>PMFIVNTNVPRASVPDGFLSELTQQLAQATGKPPQYIAVHVVPDQLMAFGGSSEPCALCSLFSIGKIGGAQNRSYSKLLCGLLAERLRISPDRVYINYYD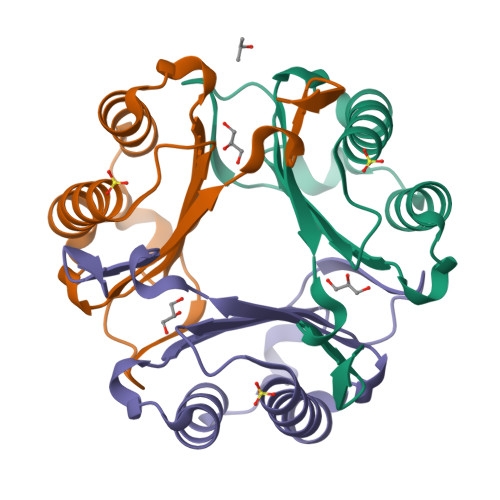MNAANVGWNNSTFA[3x]>SSRKELANAIRALSMDAVQKAKSGHPGAPMGMADIAEVLWRDFLKHNPQNPSWADRDRFVLSNGHGSMLIYSLLHLTGYDLPMEELKNFRQLHSKTPGHPE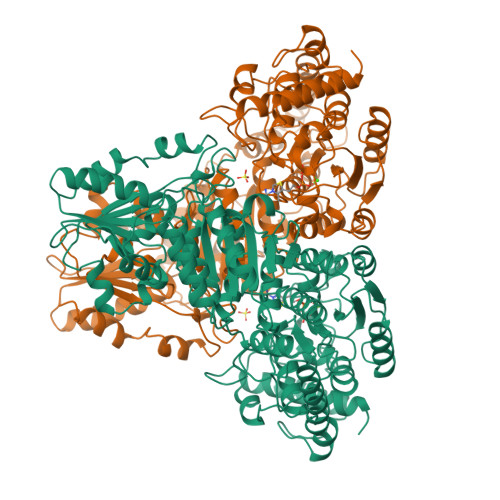VGKTAGVETTTGPLGQGIANAVGMAIAEKTLAAQFNRPGHDIVDHYTYAFMGDGCMMEGISHEVCSLAGTLKLGKLIAFYDDNGISIDGHVEGWFTDDTAMRFEAYGWHVIRDIDGHDAASIKRAVEEARAVTDKPSLLMCKTIIGFGSPNKAGTHDSHGAPLGDAEIALTREQLGWKYAPFEIPSEIYAQWDAKEAGQAKESAWNEKFAAYAKAYPQEAAEFTRRMKGEMPSDFDAKAKEFIAKLQANPAKIASRKASQNAIEAFGPLLPEFLGGSADLAPSNLTLWSGSKAINEDAAGNYIHYGVREFGMTAIANGISLHGGFLPYTSTFLMFVEYARNAVRMAALMKQRQVMVYTHDSIGLGEDGPTHQPVEQVASLRVTPNMSTWRPCDQVESAVAWKYGVERQDGPTALILSRQNLAQQERTEEQLANIARGGYVLKDCAGQPELIFIATGSEVELAVAAYEKLTAEGVKARVVSMPSTDAFDKQDAAYRESVLPKAVTARVAVEAGIADYWYKYVGLNGAIVGMTTFGESAPAELLFEEFGFTVDNVVAKAKELL[2x]>[3x]ASAWPEEKNYHQPAILNSSALRQIAEGTSISEMWQNDLQPLLIERYPGSPGSYAARQHIMQRIQRLQADWVLEIDTFLSQTPEGERSFSNIISTLNPTAKRHLVLACHYDSKYFSHWNNRVFVGATDSAVPCAMMLELARALDKKLLSLKTVSDSKPDLSL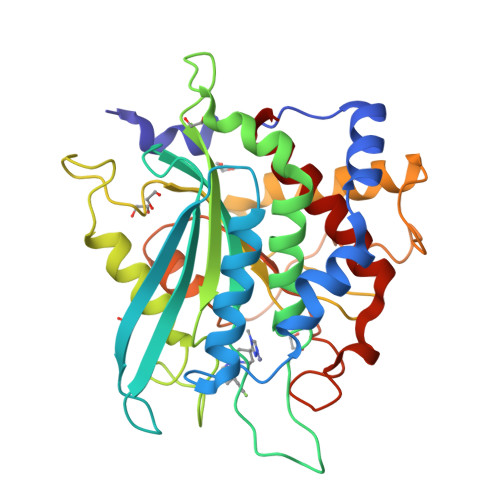QLIFFDGEEAFLHWSPQDSLYGSRHLAAKMASTPHPPGARGTSQLHGMDLLVLLDLIGAPNPTFPNFFPNSARWFERLQAIEHELHELGLLKDHSLEGRYFQNYSYGGVIQDDHIPFLRRGVPVLHLIPSPFPEVWHTMDDNEENLDESTIDNLNKILQVFVLEYLHL>GNCKPPYSFSCLIFMAIEDSPTKRLPVKDIYNWILEHFPYFANAPTGWKNSVRHNLSLNKCFKK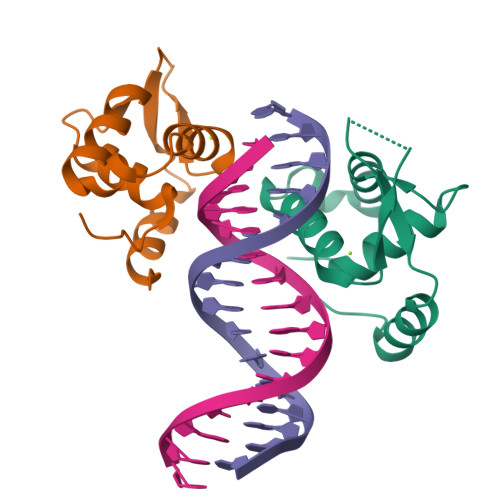VDKERSQSIGKGSLWCIDPEYRQNLIQALKKTPYHP[2x]1-(4-amino-6-methyl-1,3,5-triazin-2-yl)-N-(1H-pyrazol-3-yl)-1H-benzimidazol-2-amine 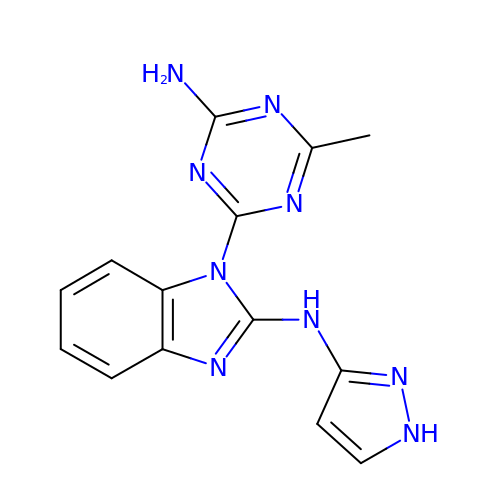| C14 H13 N9 | DMMFPXAFVNDPCA-UHFFFAOYSA-N>[2x]MTFRNCVAVDLGASSGRVMLARYERECRSLTLREIHRFNNGLHSQNGYVTWDVDSLESAIRLGLNKVCAAGIAIDSIGIDTWGVDFVLLDQQGQRVGLPVAYRDSRTNGLMAQAQQQLGKRDIYQRSGIQFLPFNTLYQLRALTEQQPELIPHIAHALLMPDYFSYRLTGKMNWEYTNATTTQLVNINSDDWDESLLAWSGANKAWFGRPTHPGNVIGHWICPQGN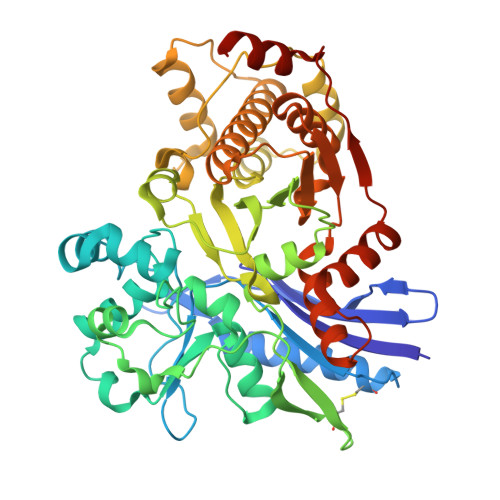EIPVVAVASHDTASAVIASPLNGSRAAYLSSGTWSLMGFESQTPFTNDTALAANITNEGGAEGRYRVLKNIMGLWLLQRVLQERQINDLPALIAATQALPACRFIINPNDDRFINPDEMCSEIQAACREMAQPIPESDAELARCIFDSLALLYADVLHELAQLRGEDFSQLHIVGGGCQNTLLNQLCADACGIRVIAGPVEASTLGNIGIQLMTLDELNNVDDFRQVVSTTANLTTFTPNPDSEIAHYVALIHSTRQTKELCA The linear ubiquitin chain assembly complex (LUBAC) regulates immune signaling, and its function is regulated by the deubiquitinases OTULIN and CYLD, which associate with the catalytic subunit HOIP. We here show that CYLD interacts with HOIP via spermatogenesis-associated protein 2 (SPATA2). SPATA2 interacts with CYLD through its non-canonical PUB domain, which binds the catalytic CYLD USP domain in a CYLD B-box-dependent manner. SPATA2 also harbors a conserved PUB-interacting motif that selectively docks into the HOIP PUB domain.

Indeed, species conservation analysis of the HOIP-interacting region in SPATA2 (aa 212–356) revealed a highly conserved putative PIM, Asp-Leu-Tyr-Thr, between amino acid residues 336 and 339, which is similar to the OTULIN PIM (Asp-Met-Tyr-Arg) (Elliott et al., 2014, Schaeffer et al., 2014). A complex crystal structure of the HOIP PUB domain with a peptide spanning the putative SPATA2 PIM sequence (aa 334–344) at 2.7 Å confirmed binding of the SPATA2 PIM to the HOIP PIM pocket. Two complexes in the asymmetric unit of the HOIP PUB-SPATA2 PIM crystals are highly similar (RMSD 0.7 Å), and while they crystallized in a distinct space group as compared to the HOIP PUB-OTULIN PIM crystals (P43 as compared to P61), the PIM peptides overlay perfectly and occupy the PIM pocket in a virtually identical manner. The major difference is the presence of Leu337 in SPATA2 instead of Met55 in OTULIN, and, indeed, the SPATA2 PIM resembles the “original” PIM sequence derived from p97 (Asp-Leu-Tyr-Gly-COO−) (Elliott et al., 2014, Schaeffer et al., 2014, Zhao et al., 2007). In contrast to p97, both SPATA2 and OTULIN constitute internal PIMs, in which residues extending C terminally make additional contacts. In the SPATA2 PIM, Asp340 forms a backbone hydrogen bond with Asn101 in HOIP, mimicking contacts of the OTULIN PIM (Elliott et al., 2014, Schaeffer et al., 2014). The structurally highly similar binding mode was also confirmed by biophysical binding measurements using fluorescently labeled PIM peptides and analyzing their binding to purified PUB domains by fluorescence polarization (FP). The SPATA2 or OTULIN PIM peptides displayed binding affinities of ∼300 nM with the HOIP PUB domain, but did not interact with PUB domains of PNGase or UBXN6 in this assay. In line with the in vitro analysis, substitution of the conserved Tyr338 in the SPATA2 PIM to Ala (Y338A) or Phe (Y338F) largely abrogated the interaction of SPATA2 with HOIP in cells, without affecting SPATA2 binding to CYLD. Moreover, co-expression of V5-tagged HOIP and SPATA2 variants showed that the SPATA2 PIM is needed to co-immunoprecipitate CYLD and HOIP, demonstrating that the CYLD-SPATA2 complex is linked to LUBAC via the SPATA2 PIM-HOIP PUB interaction.

>[2x]GEEERAFLVAREELASALRRDSGQAFSLEQLRPLLASSLPLAARYLQLDAARLVRCNAHGEPRNYLNTLSTALNILEKYGRNLLSPQRPRYWRGVKFNNPVFRSTVDAVQGGRDVLRLYGYTEEQPDGLSFPEGQEEPDEHQVATVTLEVLLLRTELSLLLQNTHPRQQALEQ;>DVDLYTDS[2x]> SEKPVYLSVKADNSMFIGNDPVTDETMITALNALTEGKKDTTIFFRADKTVDYETLMKVMDTLHQAGYL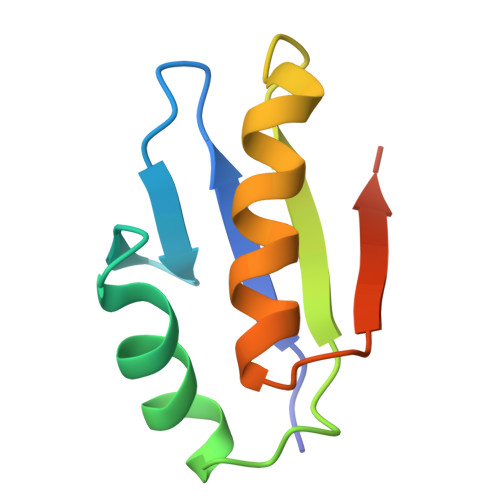KIGLVGEETAKAK>[2x]GSSHHHHHHMLDVVKGNLIVSCQALSDEPLHSSFIMGRMAIAAKQ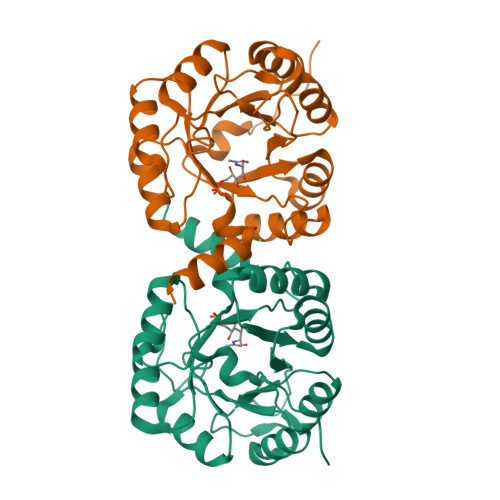GGAAAIRAQGVNDINEIKEVTKLPIIGIIARNYDDSEIYITPTMKEVDELLKTDCEMIALDATKRKRPNGENVKDLVDAIHAKGRLAMADISTLEEGIEAEKLGFDCVSTTLSGYTPYSKQSNSVDFELLEELVKTVKIPVICEGRINTPEELKKALDLGAYSAVVGGAITRPQQITKRFTDIL>[2x]MKLKSFGVFGNPIKHSKSPLIHNACFL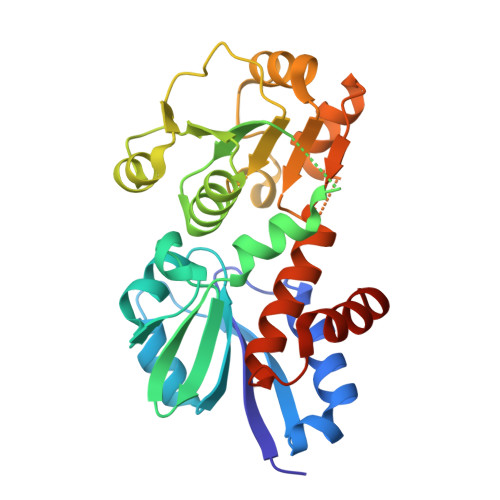TFQKELRFLGHYHPILLPLESHIKSEFLHLGLSGANVTLPFKERAFQVCDKIKGIALECGAVNTLVLENDELVGYNTDALGFYLSLKQKNYQNALILGAGGSAKALACELKKQGLQVSVLNRSSRGLDFFQRLGCDCFMEPPKSAFDLIINATSASLHNELPLNKEVLKGYFKEGKLAYDLAYGFLTPFLSLAKELKTPFQDGKDMLIYQAALSFEKFSASQIPYSKAFEVMRSVFHHHHHH(3R)-1-methylpiperidin-3-yl 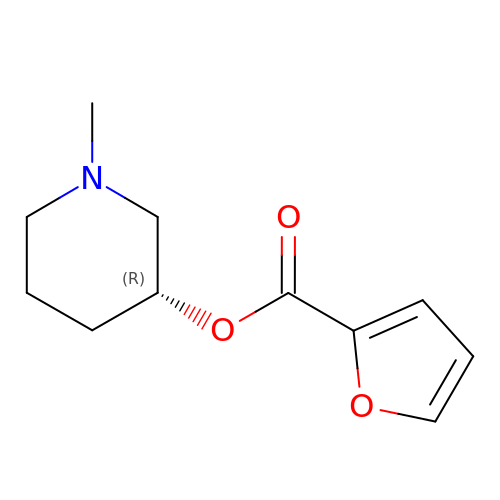furan-2-carboxylate | C11 H15 N O3 | KTNFUDPJGVBBNF-SECBINFHSA-N> MIKLGIVMDPIANINIKKDSSFAMLLEAQRRGYELHYMEMGDLYLINGEARAHTRTLNVKQNYEEWFSFVGEQDLPLADLDVILMRKDPPFDTEFIYATYILERAEEKGTLIVNKPQSLRDCNEKL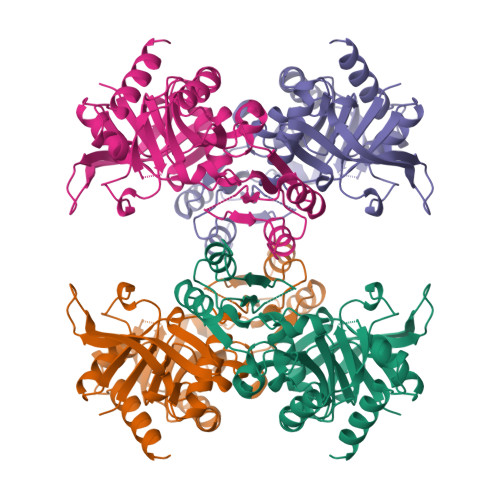FTAWFSDLTPETLVTRNKAQLKAFWEKHSDIILKPLDGMGGASIFRVKEGDPNLGVIAETLTEHGTRYCMAQNYLPAIKDGDKRVLVVDGEPVPYCLARIPQGGETRGNLAAGGRGEPRPLTESDWKIARQIGPTLKEKGLIFVGLDIIGDRLTEINVTSPTCIREIEAEFPVSITGMLMDAIEARLQQQ> HMDMRSLRVQEVPTARGMISDRSGRPLAVSVPVNAVWADPKELIEQGGISLDTRWKA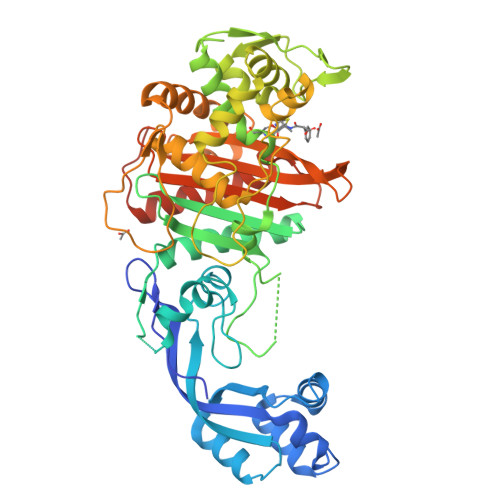LSDALEIPLDQLATRINANPKGRFVYLARQVNPAIGDYIRKLKLPGIHLRQESRRYYPAGQVMAHIIGVTNIDGQGIEGVEKSFDRWLTGQPGERTVRKDHYGRVIEDISSVDSQAAHNLVLSVDERLQALVYRELNNAVAFNKAESGTAVLVDVNTGEVLAMANSPSYNPNNLTGTPKDAMRNRAITDIFEPGSTVKPMVVMTALQHGVVKENSVLNTLPYFVNGHQIKDVARYAELSVTGILQKSSNVGVSKLALAMPSSALVDTYSRFGFGKATNLGLVGESSGLYPKKQRWSDIERATFSFGYGLMVTPLQLARVYATIGSMGVYRPLSITRVDPPVAGERIFPEPLVRTVVHMMESVALPGGGGTKAAIKGYRIAIKTGTAKKVGPDGKYMDRYLAYTAGVAPASNPRFALVVVINDPQAGKYYGGAVSAPVFGAIMGGVLRTMNIEPDALPTGDKSELVINTKEGSGGRS>KEATWVTDKPLTLKIHMHFRDKWVWDENWPVAKESFRLTNVKLQSVANKAATNSQEQFNLMMASGDLPDVVGGDNLKDKFIQYGQEGAFVPLNKLIDQYAPHIKAFFKSHPEVERAIKAPDGNIYFIPYVPDGVVARGYFIREDWLKKLNLKPPQNIDELYTVLKAFKEKDPNGNGKADEVPFIDRHPDEVFRLVNFWGARSSGSDNYMDFYIDNGRVKHPWAETAFRDGMKHVAQWYKEGLIDKEIFTRKAKAREQMFGGNLGGFTHDWFASTMTFNEGLAKTV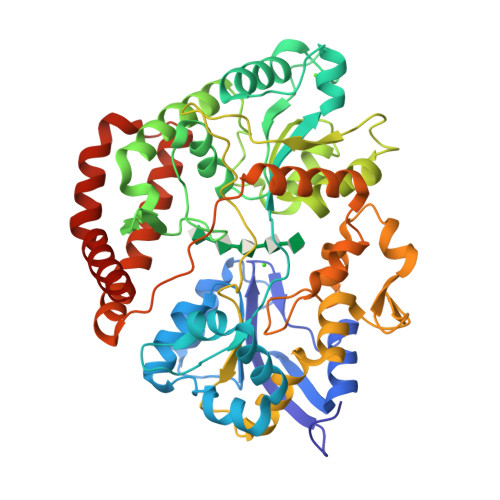PGFKLIPIAPPTNSKGQRWEEDSRQKVRPDGWAITVKNKNPVETIKFFDFYFSRPGRDISNFGVPGVTYDIKNGKAVFKDSVLKSPQPVNNQLYDMGAQIPIGFWQDYDYERQWTTPEAQAGIDMYVKGKYVMPGFEGVNMTREERAIYDKYWADVRTYMYEMGQAWVMGTKDVDKTWDEYQRQLKLRGLYQVLQMMQQAYDRQYKN[2x]> GSHMTDPSKLAVAVVDSSNMNRSMEAHNFLAKKGFNVRSYGTGERVKLPGMAFDK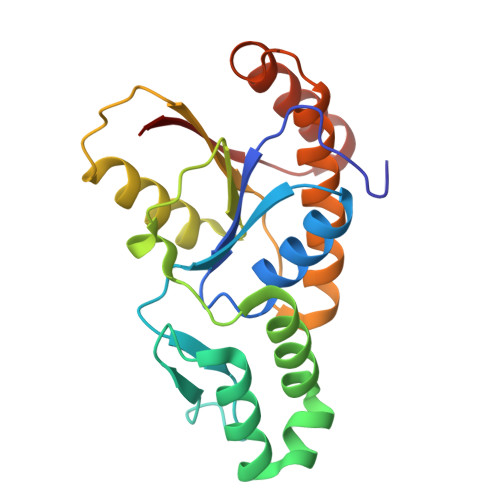PNVYEFGTKYEDIYRDLESKDKEFYTQNGLLHMLDRNRRIKKCPERFQDTKEQFDIIVTVEERVYDLVVMHMESMESVDNRPVHVLNVDVVNNAEDALMGAFVITDMINMMAKSTDLDNDIDELIQEFEERRKRVILHSVLFY alosetron | C17 H18 N4 O | 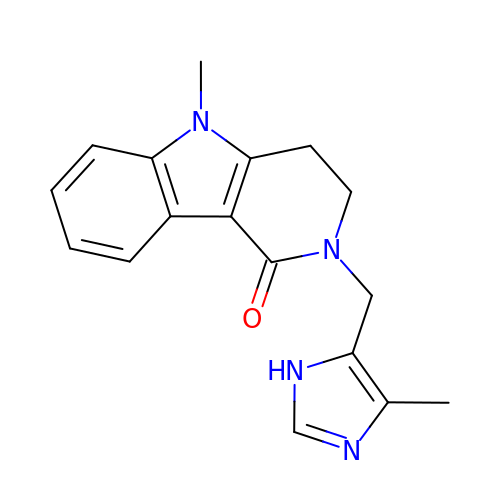JSWZEAMFRNKZNL-UHFFFAOYSA-N> AAAAAAMTMMDMNFKYCHKIMKKHSKSFSYAFDLLPEDQRKAVWAIYAVCRKIDDSIDVYGDIQFLNQIKEDI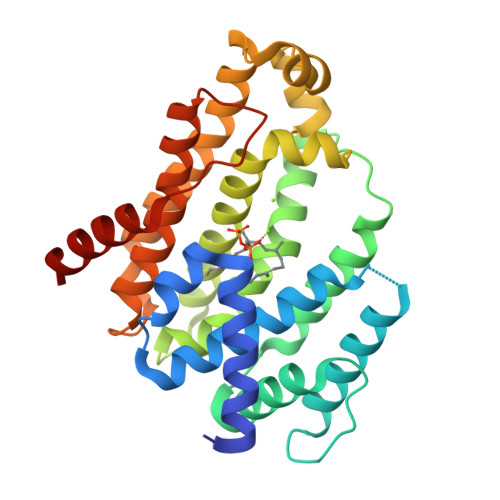QSIEKYPYEYHHFQSDRRIMMALQHVAQHKNIAFQSFYNLIDTVYKDQHFTMFETDAELFGACYGVAGTVGEVLTPILSDHETHQTYDVARRLGESLQLINILRDVGEDFENERIYFSKQRLKQYEVDIAEVYQNGVNNHYIDLWEYYAAIAEKDFRDVMDQIKVFSIEAQPIIELAARIYIEILDEVRQANYTLHERVFVEKRKKAKLFHEINSKYHRI>MEFQRVHQQLLQSHHLFEPLSPVQLQELLASSDLVNLDKGAYVFRQGEPAHAFYYLISGCVKIYRLTPEGQEKILEVTNERNTFAEAMMFMDTPNYVATAQAVVPSQLFRFSNKAYLRQLQDNTPLALALLAKLSTRLHQRIDEIETLSLKNATHRVVRYLLTLAAHAPGENCRVEIPVAKQLVAGHLSIQPETFSRIMHRLGDEGIIHLDGREIS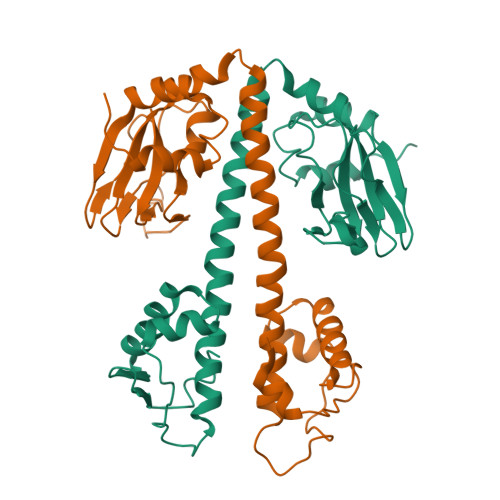ILDRERLECFE[10x]> AMRDIDSVM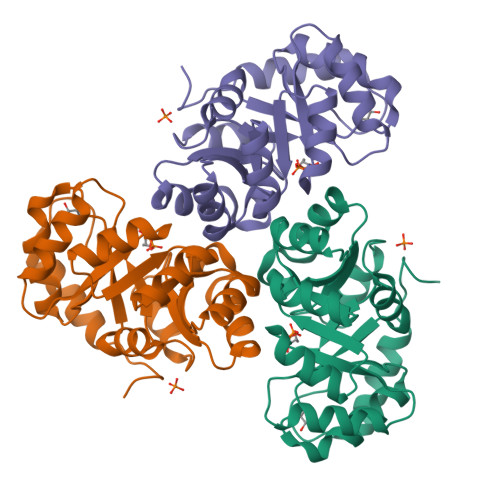RLAPVMPVLVIEDIADAKPIAEALVAGGLNVLEVTLRTPCALEAIKIMKEVPGAVVGAGTVLNAKMLDQAQEAGCEFFVSPGLTADLGKHAVAQKAALLPGVANAADVMLGLDLGLDRFKFFPAENIGGLPALKSMASVFRQVRFCPTGGITPTSAPKYLENPSILCVGGSWVVPAGKPDVAKITALAKEASAFKRAAVA>FTLLEIMVVIVILGVLASLVVPNLMGNKEKADRQKVVSDLVALEGALDMYKLDNSRYPTTEQGLQALVSAPSAEPHARNYPEGGYIRRLPQDPWGSDYQLLSPGQCGQVDIFSLGPDGV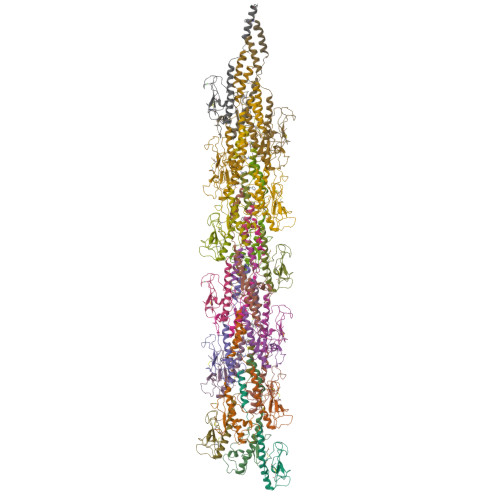PESNDDIGNCTIGKK[25x]>[2x]ELDRDPEGKDFQQPYTSFVQTKQNRDGLYALLRNTENPRMHFYQELQSDMYCTTITDGNSLAPFVNWDLGILNDHGRADEDEVSGIAGYYFVYNRLNQQANAFVNNTEAALQNQVYKNSTEIANAKSFLAEGKVLQALAIWRLMDRFSFHESVTEVNSGAKDLGVILLKEYNPGYIGPRATKAQCYDYIL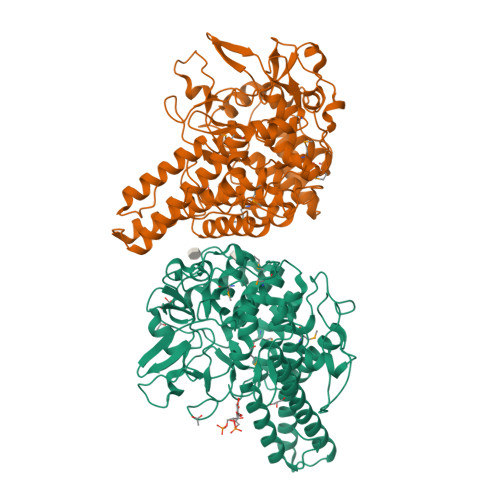SRLSEAIEVLPENRESVLYVSRDYAYALRARIYLALGEYGKAAADAKMVVDKYPLIGAADASEFENIYRSDANNPEIIFRGFASATLGSFTATTLNGAAPAGKDIKYNPSAVPFQWVVDLYENEDFRKSVYIAKVVKKDKGYLVNKFLEDKAYRDVQDKPNLKVGARYFSVAEVYLILVESALQTGDTPTAEKYLKALSKARGAEVSVVNMEALQAERTRELIGEGSRLRDMVRWSIPNNHDAFETQPGLEGFANTTPLKAQAPVGFYAYTWEFPQRDRQTNPQLIKNWPI> SGISLDNSYKMDYPEMGLCIIINNKNFHKSTGMTSRSGTDVDAANLRETFRNLKYEVRNKNDLTREEIVELMRDVSKEDHSKRSSFVCVLLSHGEEGIIFGTNGPVDLKKITNFFRGDRCRSLTGKPKLFIIQACRGTELDCGIATDSGVDDDMACHKIP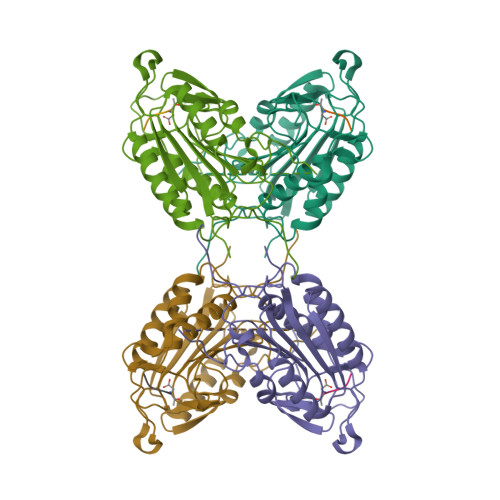VEADFLYAYSTAPGYYSWRNSKDGSWFIQSLCAMLKQYADKLEFMHILTRVNRKVATEFESFSFDATFHAKKQIPCIVSMLTKELYFYHH> GMNSNQPGLDLLGDPIVLTQRLVDIPSPSGQEKQIADEIEDALRNLNLPGVEVFRFNNNVLARTNRGLASRVMLAGH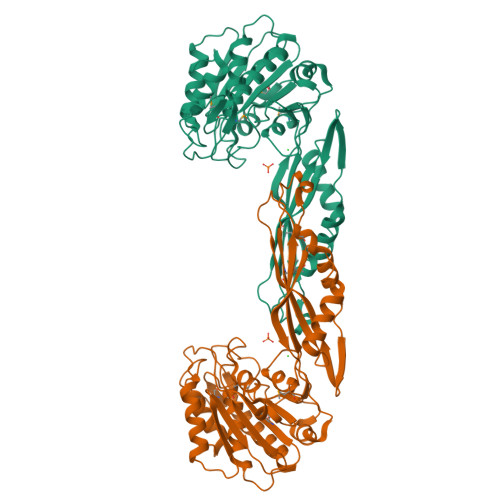IDTVPIADNLPSRVEDGIMYGCGTVDMKSGLAVYLHTFATLATSTELKHDLTLIAYECEEVADHLNGLGHIRDEHPEWLAADLALLGEPTGGWIEAGCQGNLRIKVTAHGVRAHSARSWLGDNAMHKLSPIISKVAAYKAAEVNIDGLTYREGLNIVFCESGVANNVIPDLAWMNLNFRFAPNRDLNEAIEHVVETLELDGQDGIEWAVEDGAGGALPGLGQQVTSGLIDAVGREKIRAKFGWTDVSRFSAMGIPALNFGAGDPSFAHKRDEQCPVEQITDVAAILKQYLSE(4AR,6R,7S,8R,8AR)-8-((5R,6R)-3-CARBOXY-TETRAHYDRO-4,5,6-TRIHYDROXY-2H-PYRAN-2-YLOXY)-HEXAHYDRO-6,7-DIHYDROXY-2-METHYLPYRANO[3,2-D][1,3]DIOXINE-2-CARBOXYLIC 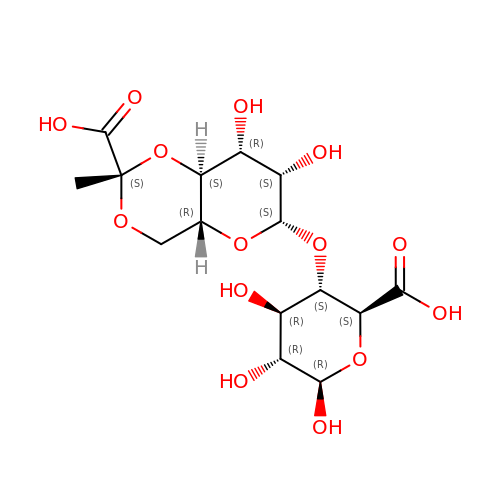ACID) | C15 H22 O14 | GZJXZKGVHLWBOW-AISSFXTFSA-N> MFEIKLNDRITEFLRKFKNSAKSNEGIDEDIDLFLKRHAIPMQSLLFYVKEYRKDSDLQCSIKELLKPLEFEFKPKAVRGLHYSEDFKKKLEFLK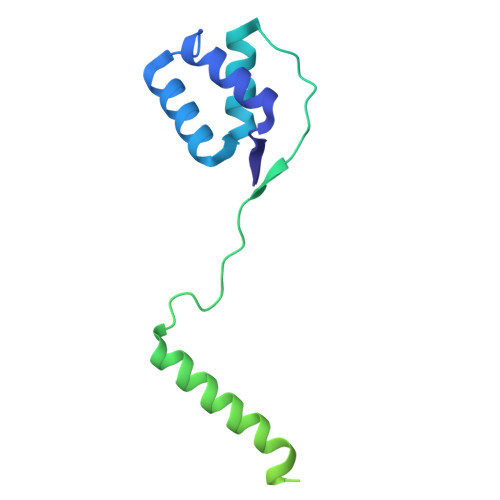YQEQELEYQSMVKRSKSVFSLQEDDELTPSQINKQIKEQVTTVFNVLVSVISVVVAIWYWTGSSTNFPVHVRLLLCLFFGILVLVADVVVYNSYLKKLEEAKVKEKTKVEKKKVLSKITL> MSSPCCVAIRRVARTTLESGRRQVDSKSTDVSPFFTGTQQMSLPSAGMVTKIRNFS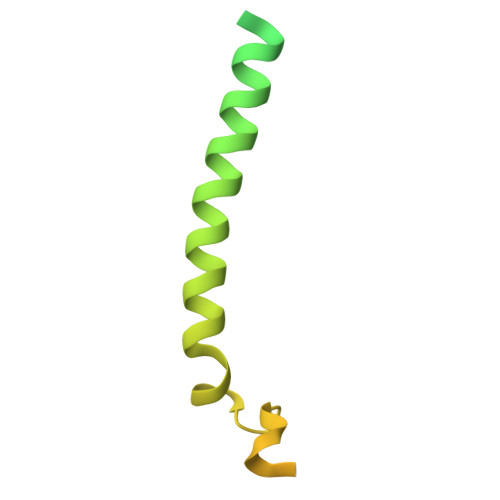SVKFMDQKRSGEETVYFKKEDEALLRNLLANHPEYDPKYSVDHMNAEVGSIARDITLACQKHGMKDPSAAFMKDLISIFGAHGYAKNSK> MNDIIIN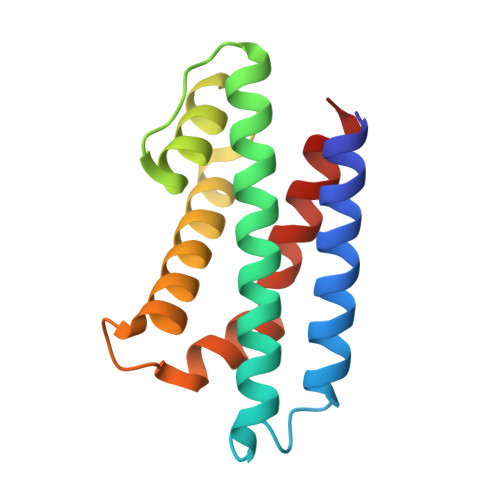KIATIKRCIKRIQQVYGDGSQFKQDFTLQDSVILNLQRCCEACIDIANHINRQQQLGIPQSSRDSFTLLAQNNLITQPLSDNLKKMVGLRNIAVHDYQELNLDIVVHVVQHHLEDFEQFIDVIKAE> MSLTDEPKLLAEPREGVPNVIDTLPAFRDYCSELASSHGSLAADAERASGFRYGHEDWLVQFKRDGAGIGLLDPQALAAAGADWNDFNRAVGDAVWILHDSLQDLPGFDELGMEPQRLFDTEIAARLLGLKRFGLAAVTEHFLGLTLAKEHSAADWSYRPLPRDWRNYAALDVELLIELETKMRAELKRQGKMEWAQEEFDYALKEGLGPRKEHLIPWMHVSHITEVMRDRQALAIVRALWTRRDELAREYDIAPTLLLSDSSIIE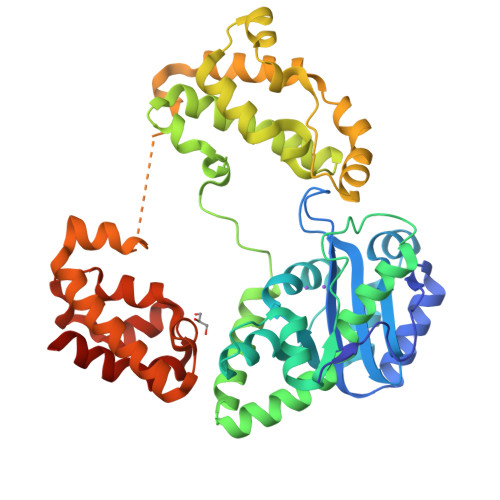VAKRKPHNAAQFRSIRSINERVRIHTDSEQDKMFERYAPIQRKIKPSMWKNIIQDALALPPSEWPDVDGGAARRHESQSASAPKSIRVWKERYPERLQVLNRVRKAVSQIAEDTRTPVEIVIKPQYLRNLCWTDEPRKRDVARFLSEQGARDWQVSLVAESVSRAIEGHHHHHH>[2x]MHHHHHHYFSINDSKILSLQNKKNTLMDTSGYNAEVRVEGNVQLNPIFPFDFKLGSSGDDRGKVIVTQNENIVYNAMYESFSISFWIRINK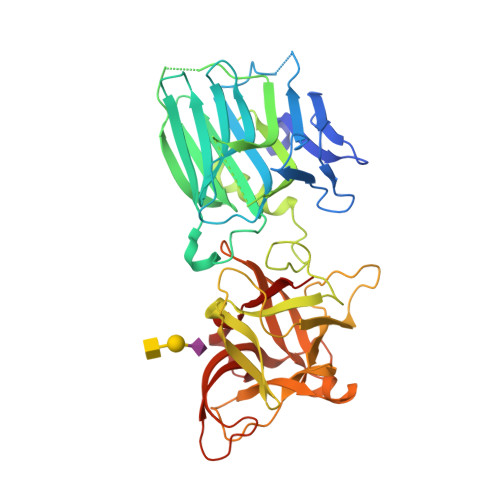WVSNLPGYTIIDSVKNNSGWSIGIISNFLVFTLKQNENSEQDINFSYDISKNAAGYNKWFFVTITTNMMGNMMIYINGKLIDTIKVKELTGINFSKTITFQMNKIPNTGLITSDSDNINMWIRDFYIFAKELDDKDINILFNSLQYTNVVKDYWGNDLRYDKEYYMINVNYMNRYMSKKGNGIVFNTRKNNNDFNEGYKIIIKRIRGNTNDTRVRGENVLYFNTTIDNKQYSLGMYKPSRNLGTDLVPLGALDQPMDEIRKYGSFIIQPCNTFDYYASQLFLSSNATTNRLGILSIGSYSFKLGDDYWFNHEYLIPVIKIEHYASLLESTSTHWVFVPAS Recently, the bacterial strain Ideonella sakaiensis 201-F6 was discovered and shown to grow on low-crystallinity PET films. Two α/β-hydrolase fold enzymes (α/β-hydrolases), PETase and MHETase, work together to degrade PET in two steps via MHET, yielding TPA and ethylene glycol—the building blocks required for a new round of PET synthesis. We have determined crystal structures of recombinantly expressed and purified I. sakaiensis MHETase in its ligand-free form (2.05 Å resolution), MHETase bound to a nonhydrolyzable mono-(2-hydroxyethyl) terephthalamide (MHETA, 2.1 Å resolution) or to benzoic acid (BA, 2.2 Å resolution) as well as ligand-free PETase (2.0 Å resolution) (2a−f). PETase and MHETase only share the α/β-hydrolase fold (2.87 Å RMSD for 184 out of 262 residues aligned).

The main chain conformation in the MHETase-MHETA complex structure is nearly identical to that of MHETase without substrate (RMSD 0.54 Å) and sheds light on the positioning of MHET for catalysis. While the catalytic triad and oxyanion hole residues are part of the α/β-hydrolase domain, substrate specificity is almost exclusively conferred by the lid domain. Hydrophobic contacts between the phenyl ring of MHETA and the α/β-hydrolase domain are restricted to primarily F495, and to a lesser extent G132 and A494. Strikingly, MHETA is tightly bound by the lid domain residues F415, L254 and W397 surrounding nearly the entire MHETA phenyl moiety. The two oxygens of the free carboxylate make contacts to R411, which is held in place by S416, S419 and the backbone amide of G258, which maintain a hydrogen bond network involving three water molecules. Despite their overall high similarity, a detailed comparison of MHETase structures in the absence and presence of the substrate reveals an induced-fit mechanism upon MHETA binding. In the ligand-free structure, F415 points away from the active site and thus opens it for substrate binding. The association of MHETA then triggers a near 180° rotation of the F415 side chain around χ1, closing the active site and consolidating the interaction. Our structural analysis suggests that R411 enforces a strictly required negative charge in the 4-position to the hydrolyzed ester bond, which clearly explains why diesters and diamides show no binding to MHETase. Thus, substrate recognition strongly relies on the aromatic ring as well as the carboxylate function of MHET both guiding its positioning for hydrolysis.

>[6x]MNHKVHHHHHHMGGGSTPLPLPQQQPPQQEPPPPPVPLASRAACEALKDGNGDMVWPNAATVVEVAAWRDAAPATASAAALPEHCEVSGAIAKRTGIDGYPYEIKFRLRMPAEWNGRFFMEGGSGTNGSLSAATGSIGGGQIASALSRNFATIATDGGHDNAVNDNPDALGTVAFGLDPQARLDMGYNSYDQVTQAGKAAVARFYGRAADKSYFIGCSEGGREGMMLSQRFPSHYDGIVAGAPGYQLPKAGISGAWTTQSLAPAAVGLDAQGVPLINKSFSDADLHLLSQAILGTCDALDGLADGIVDNYRACQAAFDPATAANPANGQALQCVGAKTADCLSPVQVTAIKRAMAGPVNSAGTPLYNRWAWDAGMSGLSGTTYNQGWRSWWLGSFNSSANNAQRVSGFSARSWLVDFATPPEPMPMTQVAARMMKFDFDIDPLKIWATSGQFTQSSMDWHGATSTDLAAFRDRGGKMILYHGMSDAAFSALDTADYYERLGAAMPGAAGFARLFLVPGMNHCSGGPGTDRFDMLTPLVAWVERGEAPDQISAWSGTPGYFGVAARTRPLCPYPQIARYKGSGDINTEANFACAAPP> DVSFRLSGADPRSYGMFIKDLRNALPFREKVYNIPLLLPSVSGAGRYLLMHLFNRDGKTIT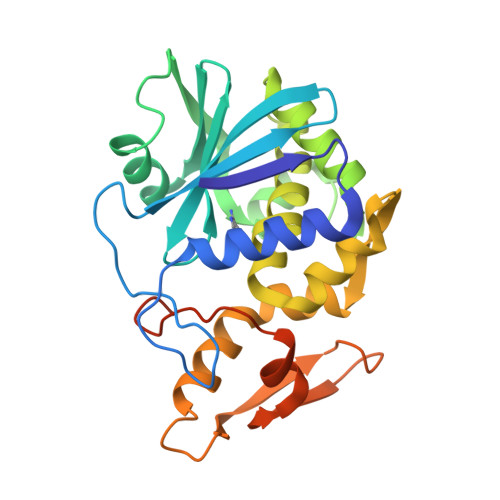VAVDVTNIYIMGYLADTTSYFFNEPAAELASQYVFRDARRKITLPYSGDYERLQIAAGKPREKIPIGLPALDSAISTLLHYDSTAAAGALLVLIQTTAEAARFKYIEQQIQERAYRDEVPSLATISLENSWSGLSKQIQLAQGNNGIFRTPIVLVDNKGNRVQITNVTSKVVTSNIQLLLNTRNIAEGDNGDVSTTHGFSSY> MGSANGKTLGEVWKRELNLLD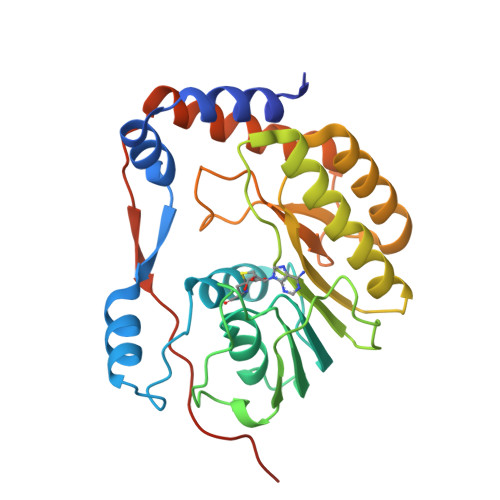KRQFELYKRTDIVEVDRDTARRHLAEGKVDTGVAVSRGTAKLRWFHERGYVKLEGRVIDLGCGRGGWCYYAAAQKEVSGVKGFTLGRDGHEKPMNVQSLGWNIITFKDKTDIHRLEPVKCDTLLCDIGESSSSSVTEGERTVRVLDTVEKWLACGVDNFCVKVLAPYMPDVLEKLELLQRRFGGTVIRNPLSRNSTHEMYYVSGARSNVTFTVNQTSRLLMRRMRRPTGKVTLEADVILPIGTRSVGSSSHHHHHH>MWSHPAVRKSSSKTIRSRSIWDDAHAMLEKAKAEGISTVWDRAAEQTPACKFCELGTTCRNCIMGPCRIANRKDGKMRLG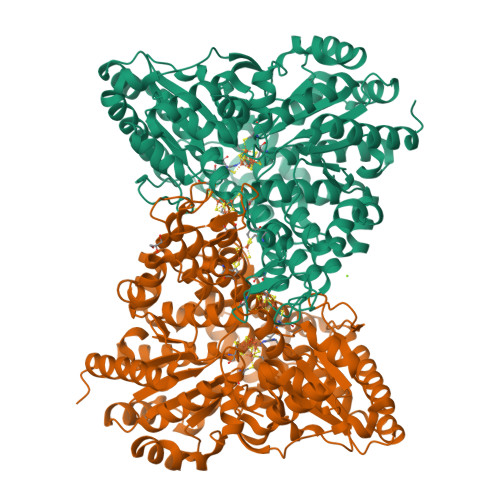VCGADADVIVARNFGRFIAGGAAGHSDHGRDLIETLEAVAEGKAPGYTIRDVAKLRRIAAELGVADAATRPAHDVAADLVTICYNDFGSRRNALAFLARAPQVRRDLWQRLGMTPRGVDREIAEMMHRTHMGCDNDHTSLLVHAARTALADGWGGSMIGTELSDILFGTPRPRQSTVNLGVLRKDAVNILVHGHNPVVSEMILAATREPAVRQAAQDAGAADINVAGLSCTGNELLMRQGIPMAGNHLMTELAIVTGAADAIVADYQCIMPSLVQIAACYHTRFVTTSPKGRFTGATHVEVHPHNAQERCREIVMLAIDAYTRRDPARVDIPSQPVSIMSGFSNEAILEALGGTPKPLIDAVVAGQIRGFVGIVGCNNPKIRQDSANVTLTRELIRRDIMVLATGCVTTAAGKAGLLVPEAASKAGEGLAAVCRSLGVPPVLHMGSCVDNSRILQLCALLATTLGVDISDLPVGASSPEWYSEKAAAIAMYAVASGIPTHLGLPPNILGSENVTAMALHGLQDVVGAAFMVEPDPVKAADMLEAHIVARRARLGLTS[4x]>GIDPFTMTPSEDFVVTDRGGIVENSHRVHAAVVDAKGRLLYALGNPTRMTLARSAAKPAQALAILETEGVAGYGFDDADIALMCASHSSEDRHIARTRAMLSKIKAEEADLRCGGHPSLSEMVNRSWIKQDFIPTAVCSNCSGKAVGMLAGARAIGAGTDGYHLPDHPMQGRVKRTVAELCDLDAGDVEWGTDGCNLPTPAFPLDRLGRIYAKLASAADGSDAGEGQSTRCAALAHIFRAMARHPEMVAGEGRYCTMLMRAFDGALVGKLGADASYAIGVRASDATRQLGTDGALGISVKIEDGNLEMLYAVVTELLERLGIGSPDVRSQLASFHHPQRVNTMGVTTGGVSFPFKLRGSKSNVDDPRLAAVAR[4x]

Asparaginases (EC 3.5.1.1), which split L-asparagine to L-aspartate and ammonia, are grouped into three unrelated structural classes: Class 1 (bacterial-type), Class 2 (plant-type), and Class 3 (Rhizobium etli-type). ReAV is a homodimer with an α/β protomeric fold, formed by two tightly packed domains. The active site of the enzyme is located in a cleft on the protomer surface and marked by a zinc ion with an unusual coordination sphere created by Cys135, Lys138, Cys189, and a water molecule. The conspicuous catalytic center of the enzyme comprises two Ser-Lys tandems (Ser48-Lys51 and Ser80-Lys263), centered around the curiously hydrated Ser48 residue and located in the close vicinity of the metal binding site.

The introduction of alanine at position 139 resulted in only minor atomic shifts and structural rearrangements in the active site area, almost identical in the four protein chains. The substitution of His139 by alanine does not affect the conformation of the neighboring residues: just two water molecules, marking the sites of the two N atoms of the imidazole ring, fill the available space left by the histidine side chain, maintaining the original pattern of hydrogen bonds in the active site area. The fully occupied Zn2+ binding site is conserved in the mutant structure, as are the catalytic Ser-Lys tandems. In the close vicinity of the Ser48 hydroxyl, high difference electron density peaks were detected, previously also observed in the WT protein structure and interpreted as three closely spaced water molecules. Therefore, a water triad was modeled forming very strong H-bonds with the Ser48 Oγ atom, with O…O distances of 2.3–2.4 Å. The crystal structure of ReAV H139A shows alternative conformations of Asp187 in protein chain B. The major rotamer of Asp187 (refined occupancy 0.7) is rotated toward the side chain of Arg47, forming an H-bond to its Nε atom, as well as to the water molecule from the zinc coordination sphere and the Oγ atom of Thr341. Despite the mutation of the highly conserved His139, the H139A mutein retained the L-asparaginase activity. Interestingly, the H139A mutant matches the WT form in kcat (445 s−1 vs. 416 s−1), but its substrate specificity is reduced more than twice (5.6 mM vs. 2.7 mM). We also could not titrate the H139A mutant with Zn2+ because, as revealed by the crystal structure, it is already fully saturated with zinc. Intriguingly, the side chain of Cys249 did not undergo oxidative modification in the H139A mutant structure either, in contrast to what had been observed previously when the zinc cation was present in the WT protein structure.>PGMDSLPNPYLQSVSLTVCYMVKIKANLLSPFGKNPELQVDFGTGTGQGGDIPFRFWYCDGIVVMNTLKDGSWGKE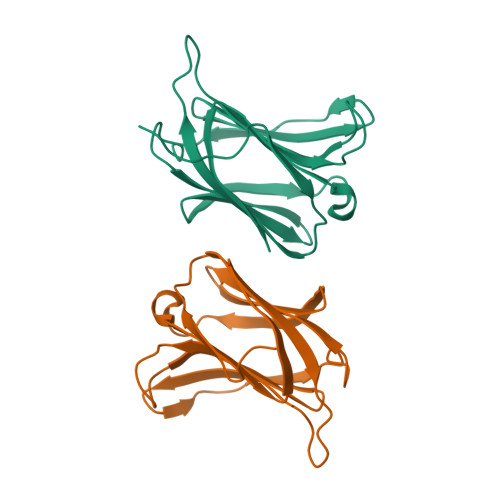QKLHTEAFVPGQPFELQFLVLENEYQVFVNNKPICQFAHRLPLQSVKMLDVRGDIVLTSVDTL[8x]>MDEGMWLMQQLGRKYAQMKERGLKMKEYDLYNPNGTSLKDAVVLFDGGCTGEVVSDRGLVLTNHHCGYDMIQAHSTLEHNYLENGFWAMREADELPNKDISVVFIDKIEDVTDYVKKELKAIKDPNSMDYLSPKYLQKLADKKAGKNFSAKNPGLSVEIKAFYGGNLYLMFTKKTYTDVRLVGAPPSSIGKFGADTDNWIWPRHTGDFSIFRIYADKNGNPAPYSEDNVPLKPKRFFNISLGGVQENDYAMIMGFPGTTHRYFTASEVDEWKSIDNDIRIRMRDIRQGVMLREMLADPQIKIMYSAKYAASQNAYKRAIGANWAIKTRGLRQNKQAMQDRLIAWGAKQGTPRYEEAVHEIDATVAKRADLRRRYWMIEEGIIRGIEFARSPIPTEDETKALQGNDASARKEAIDKIRTRYSKFANKDYSAEVDKKVAVAMLTEYLKEIPYENLPLHLRLVKDRFAGDVQAYVDDIFARSVFGSEAQFDAFAAVPSVEKLAE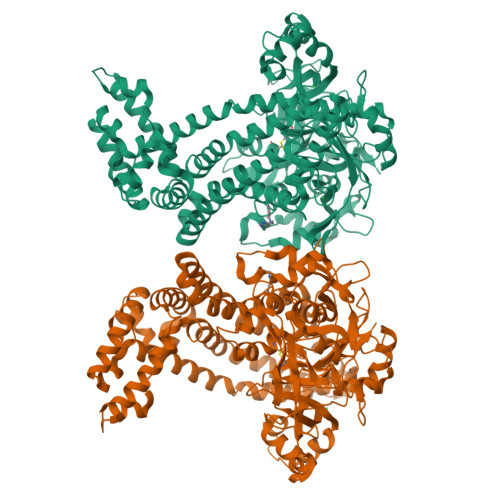DPMVLFASSVFDEYRKLYNELRPYDDPILRAQRTYIAGLLEMDGDQDQFPDANLTLRFTYGQVKGYSPRDNVYYGHQTTLDGVMEKEDPDNWEFVVDPKLKAVYERKDFGRYADRSGRMPVAFCATTHTTGGNSGSPVMNANGELIGLNFDRNWEGVGGDIQYLADYQRSIIVDIRYVLLVIDKVGGCQRLLDEMNIVPAHHHHHH[2x]> MHHHHHHETTVFLSNRSQAVRLPKAVALPENVKRVEVIA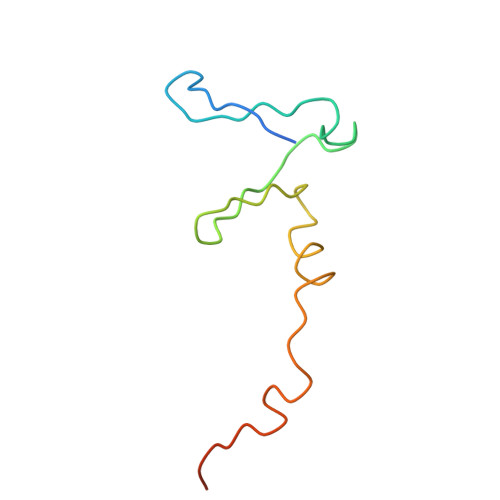VGRTRIITPAGETWDEWFDGHSVSTDFMDNREQPGMQERESF>GSTLSLTTGTDTLTGTANNDTFVAGEVAGAATLTVGDTLSGGAGTDVLNWVQAAAVTALPTGVTISGIETMNVTSGAAITLNTSSGVTGLTALNTNTSGAAQTVTAGAGQNLTATTAAQAANNVAVDGGANVTVASTGVTSGTTTVGANSAASGTVSVSVANSSTTTTGAIAVTGGTAVTVAQTAGNAVNTTLTQADVTVTGNSSTTAVTVTQTAAATAGATVAGRVNGAVTITDSAAASATTAGKIATVTLGSFGAATIDSSALTTVNLSGTGTSLGIGRGALTATPTANTLTLNVNGLTTTGAITDSEAAADDGFTTINIAGSTASSTIASLVAADATTLNISGDARVTITSHTAAALTGITVTNSVGATLGAELATGLVFTGGAGADSILLGATTKAIVMGAGDDTVTVSSATLGAGGSVNGGDGTDVLVANVNGSSFSADPAFGGFETLRVAGAAAQGSHNANGFTALQLGATAGATTFTNVAVNVGLTVLAAPTGTTTVTLANATGTSDVFNLTLSSSAALAAGTVALAGVETVNIAATDTNTTAHVDTLTLQATSAKSIVVTGNAGLNLTNTGNTAVTSFDASAVTGTGSAVTFVSANTTVGEVVTIRGGAGADSLTGSATANDTIIGGAGADTLVYTGGTDTFTGGTGADIFDINAIGTSTAFVTITDAAVGDKLDLVGISTNGAIADGAFGAAVT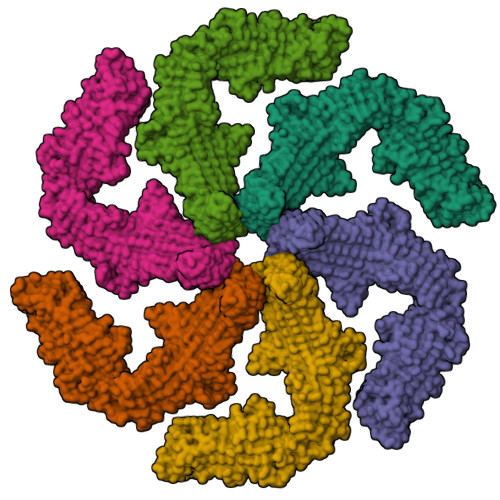LGAAATLAQYLDAAAAGDGSGTSVAKWFQFGGDTYVVVDSSAGATFVSGADAVIKLTGLVTLTTSAFATEVLTLA[6x]(2R)-N-(pyridin-2-yl)-1,4-dioxane-2-carboxamide 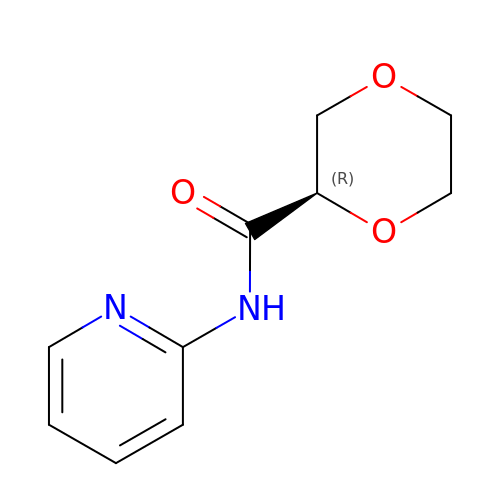| C10 H12 N2 O3 | MYQOETKNJQIOKN-MRVPVSSYSA-N> MTLGRRLACLFLACVLPALLLGGTALASEIVGGRRARPHAWPFMVSLQLRGGHFCGATLIAPNFVMSAAHCVANVNVRAVRVVLGAHNLSRREPTRQVFAVQRIFENGYDPVNLLNDIVILQLNGSATINANVQVAQLPAQGRRLGNGVQCLAMGWGLLGRNRGIASVLQELNVTVVTSLCRRSNVCTLVRGRQAGVCFGDSGSP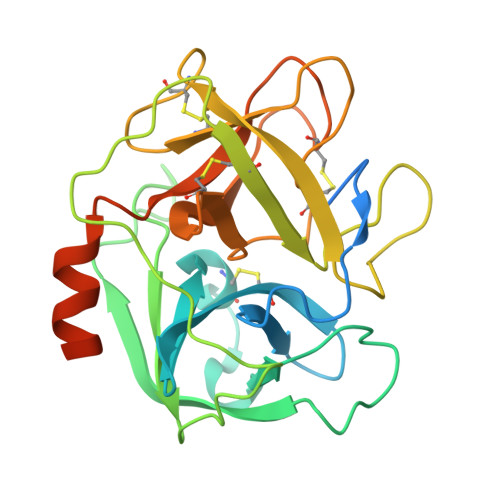LVCNGLIHGIASFVRGGCASGLYPDAFAPVAQFVNWIDSIIQRSEDNPCPHPRDPDPASRTH> GSEDRDPTQFEERHLKFLQQLGKGNFGSVEMCRYDPLQDNTGEVVAVKKLQHSTEEHLRDFEREIEILKSLQHDNIVKYKGVCYSAGRRNLKLIMEYLPYGSLRDYLQKHKERIDHIKLLQYTSQICKGMEYLGTKRYI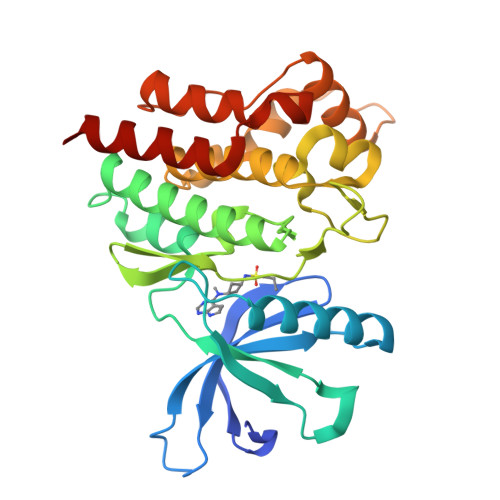HRDLATRNILVENENRVKIGDFGLTKVLPQDKEYYKVKEPGESPIFWYAPESLTESKFSVASDVWSFGVVLYELFTYIEKSKSPPAEFMRMIGNDKQGQSIVTHLIELLKNNGRLPRPDGCPDEIYMIMTECWNNNVNQRPSFRDLALRVDQIRDNMAG> RVLLALHDRAPQLKISDDRLTVVGEKGYSMVRASHGVRKGA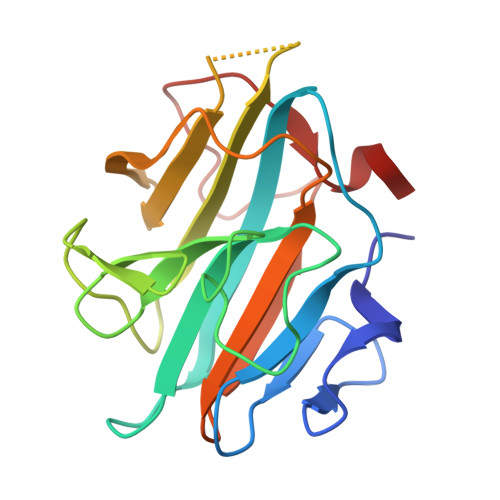WYFEITVDEMPPDTAARLGWSQPLGNLQAPLGYDKFSYSWRSKKGTKFHQSIGKHYSSGYGQGDVLGFYINLPEDISGRGSEIIFYKNGVNQGVAYKDIFEGVYFPAISLYKSCTVSINFGPCFKYPPKDLTYRPMSDMG> GPLGSGTSTAQGILQQINTILRRNNAREIEDVHNLLALDFATENQNFRYWLQTHDMFFAARQYTFHDDRSNPTNDRHDFAITSVGVDGNQND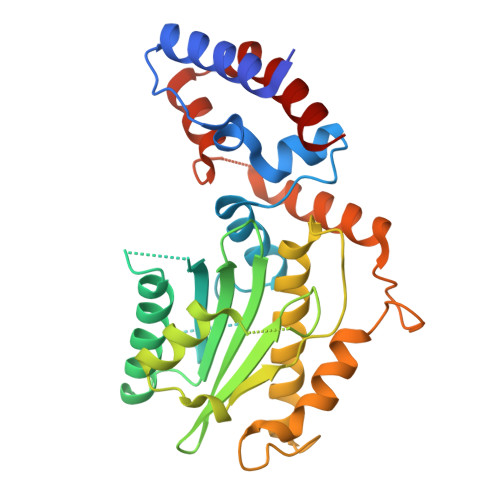PTGRDLLSSNIDNFKQKVDSGEKDRLTAIINVGNRHWVTLVIVHQNGNYYGYYADSLGPDSRIDNNIRGALRECDISDDNVHDVSVHQQTDGHNCGIWAYENARDINQAIDQALQGNSNFGEKGEGIIGYIRGLLSAGIGNDTRQPQRNEQYFRNRRRNISQLFQNDSLSSPRGRLIQGRPGIQHEIDPLLLQFLELQYPQ>[2x]SHMSKIKGNVKWFNESKGFGFI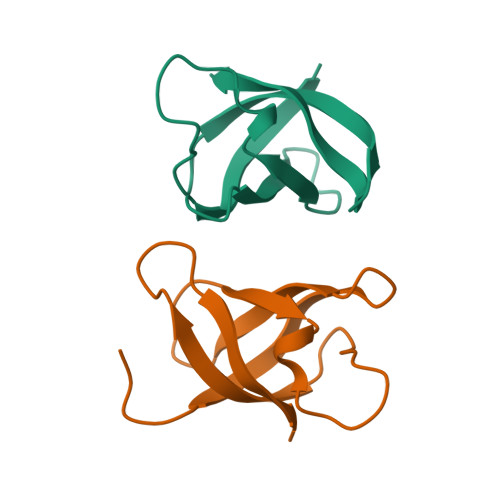TPEDGSKDVFVHFSAIQTNGFKTLAEGQRVEFEITNGAKGPSAANVTAL Phospholipid PG(16:0/cy17:0) | C39 H75 O10 P | 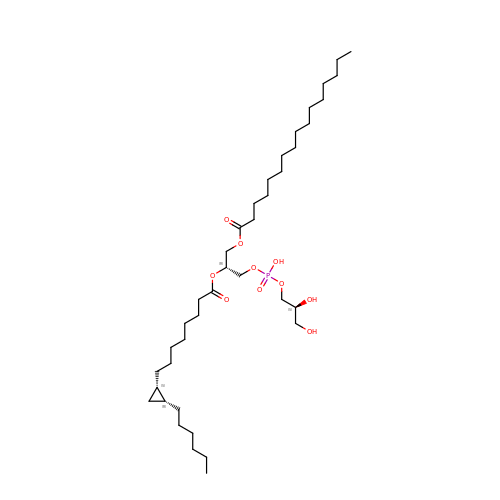JWIOKCJPLNKYBQ-TWHRXLCVSA-N3,7,11,15-TETRAMETHYL-HEXADECAN-1-OL | C20 H42 O | 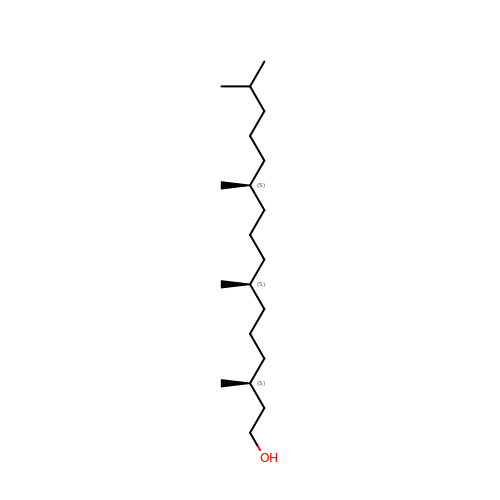AJAKLDUGVSKVDG-UFYCRDLUSA-N Riboswitches are cis-acting gene regulatory elements that are mostly found in bacteria (Lee et al., 2009). They are located in the 5′ untranslated region (UTR) of mRNAs and consist of an aptamer domain that binds the ligand, and an expression platform that controls the expression of the downstream gene. The GRA was derived by a point mutation from the guanine riboswitch (C74U) (Gilbert et al., 2006b). As a result, the specificity of the guanine riboswitch was altered to be adenine responsive, thus generating a new adenine riboswitch (GRA).

N6-methyladenine was the weakest ligand in the test set. It obtained the least favorable score of all ligands, even lower than many of the decoys. However, 15 is also the largest molecule of all binders and thus requires the largest amount of space in the binding pocket. In the predicted binding mode, the ligand adopts a conformation distinct from adenine with the N6-methylamino group pointing into the cleft between U51 and U74 resulting in unfavorable interactions (not shown). In order to adopt a similar binding mode as adenine the structural water molecule W364 would have to be expelled from the receptor. This prompted us to determine the crystal structure of the N6-methyladenine-riboswitch complex. The crystallographic analysis revealed that 15 indeed expels W364 from the binding site and adopts a similar binding mode as adenine. When docked into the receptor without the water molecule present the correct binding mode was obtained (rmsd = 0.5Å). With a score of −32.83 kJ/mol the ligand would rank third in the database screen.

> GAACAUAUAAUCGCGUGGAUAUGGCACGCAAGUUUCUACCGGGCACCGUAAAUGUCCGAUUAUGUCC> SSMEIRVRVEKDPELGFSISGGVGGRGNPFRP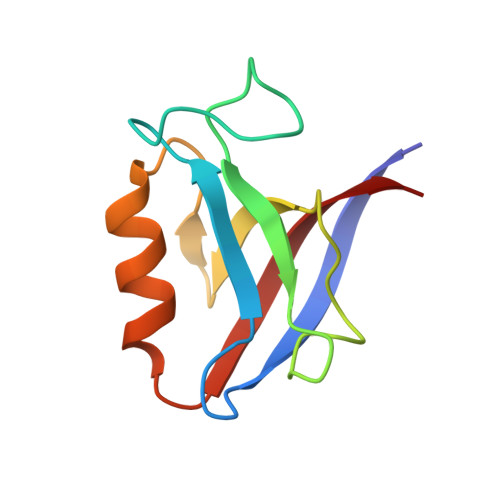DDDGIFVTRVQPEGPASKLLQPGDKIIQANGYSFINIEHGQAVSLLKTFQNTVELIIVREV> MERTFTPNVMQPTPLLPTTNDGRVTFGEAFNDLKDLARRYQLYWEGTILEGNLRAIRRNSALVQLPLYPHGLRIQPDVNNPIWNIMRDGHIPVISSGFRYFRGGLRLRIVVEGLNSCVWVQHHPDRPSIFSRPIIGRYIAAKDAYRNHAYAAYVQNMSVNRTIEVEVPFYQPGLYGMLNASDNNTANSFDRLRFTGLGDLLIGIEGEQPIPKEGIEISVYYSIADDFSF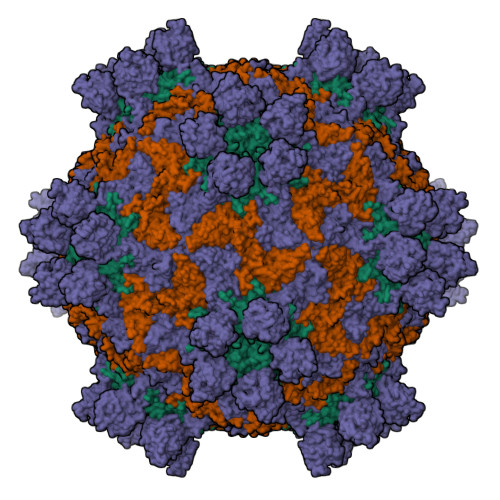NIFCGFPPMVYCDETYSAATPDLAQYFEDEVTIAQPE;> MDRPEGSEERTVQTSNVVLGETNIESQDIASKEYSPTWDRLASSEVSDEYPMLTDRWLFWKSVKWEVNDSAFGKMLVQEKFPQSWVQMDVNVNNIPRYTNIPNFIPFNIHQYMRADFEVKIYVNPNDFVSGWLIMAFLYQGSEMFDYKLRRNPAALMQMPHVLVNVGAANEATLKIPYRYVRPFMRCKDILRGDNLITGVTEPLNMGVLFVEVLIPFRTSAASSAPKSLDVSLFVKMTNAKFTGMVDGSIALLSKPIALPE;> DNPPDPTPAKFFVPIPSHSWAHGTNTSEPTNTLRLDGGVVGVGRSDDIGTSDTAISGIIGVYGLLKPFDWNANDTGRNVGGHLLWSMPVHPQVDKDQVIQVMTQSKLTQYYLPPISVVSSLYAYTRGSIKYKFLFGNNPRHNARLLVAYIPGISSDNRLTLERARNSAHVVFSLNEVSEFVFTVPYITDTMWWPRKYGGPQAAGEFVAPSYICMFILNPLVAMESVPSIVTIVPMIAAGDDFEVAVPAQPAVGLSRNIDVIYPKDSIISFKSGYFPVYVGSWHSFFDSTKAILRYGAVSDHIAQLGNIPANVNRKAFWIVVGDTIKFKTKLDKINGTEWFIPEGEYTLGYGVVWRDGAYAYMVPYPLTPLGEKIAQYTASLLASNTAISQIRPYIPDYIVDSAASKDNILWSPIEDRLRAQTEWVMAEPE>MISGLSHITLIV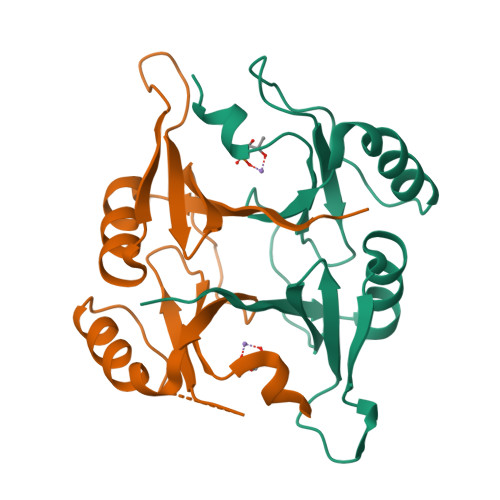KDLNKTTAFLQNIFNAEEIYSSGDKTFSLSKEKFFLIAGLWICIMEGDSLQERTYNHIAFQIQSEEVDEYTERIKALGVEMKPERPRVQGEGRSIYFYDFDNHLFELHAGTLEQRLKRYHE[6x]>KTVQVTLHAVETDVAYDNKGSTYRAWTFDGKVPGPVVRVTEGDTVEFTLINDKNSKNSHSMDFHAARLDVVEDFESIKPGETKKYTFTADNPGVFFYHCGSDPMIQHIARGMYGVIIVDPKDANALPKADREYVLIQAEHYENPDDKTAMMQNKWSNVVFNGGVFKYDPVHDSEATSWLQAKPGERVRIYFVNAGPNELSSLHPIAGIWDRVYPSGNPKNVQYALQSYLIGAGDAATLDLISPVEGANAIVDHSMRHAHSGAIAVIMFTNDADPEAGRG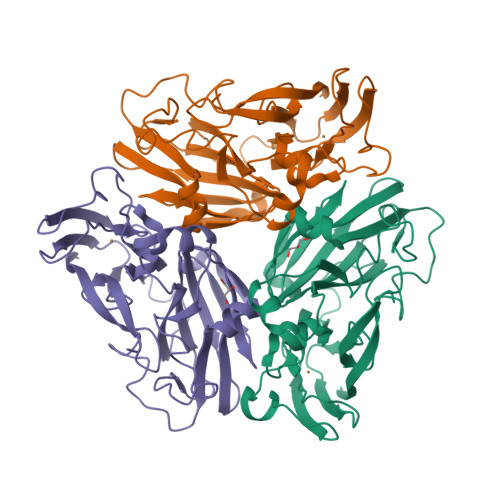ENILIR[6x]The TRAPP complexes are nucleotide exchange factors that play essential roles in membrane traffic and autophagy. TRAPPII activates Rab11, and TRAPPIII activates Rab1, with the two complexes sharing a core of small subunits that affect nucleotide exchange but being distinguished by specific large subunits that are essential for activity in vivo. We report a cryo‐EM structure of the entire Drosophila TRAPPIII complex. The TRAPPIII‐specific subunits TRAPPC8 and TRAPPC11 hold the catalytic core like a pair of tongs, with TRAPPC12 and TRAPPC13 positioned at the joint between them.

The overall shape of the complex is that of two arched arms connected at one vertex with TRAPPC12 and TRAPPC13, and then spreading apart to hold the core between their other ends like a pair of tongs. Overall, we were able to model the core, and the N‐terminal halves of TRAPPC8 and TRAPPC11. The C‐terminal halves of these subunits, along with TRAPPC12 and TRAPPC13, were unmodelled as although helices were recognisable in many regions, the sequences could not be attributed. The primary interactions between the core and the arms are via binding of TRAPPC2 and TRAPPC2L to TRAPPC8 and TRAPPC11, respectively. Two additional points of interaction between the arms and the core are visible in the TRAPPIII map as indicated by continuous densities between the flat surface of the core and the middle regions of both TRAPPC8 and TRAPPC11. TRAPPC8 is linked to density formed by the connection of the first two α‐helices of TRAPPC3b and TRAPPC5. Similarly, density from TRAPPC11 connects to a region formed by the first two α‐helices of TRAPPC3a and TRAPPC6. We detected 146 total cross‐links, and 75 of them mapped to residues present in the structural model—32 cross‐links were inter‐molecular and 43 intra‐molecular. None of these cross‐links exceeded the maximum distance constraint for disuccinimidyl dibutyric urea (DSBU) of ~30 Å, thus providing good validation for the atomic model of the TRAPPIII complex (Appendix Fig S5B and Table EV1). The TRAPPC8 arm is positioned such that it would contact Rab1 that is bound to the core, indicating how the arm could determine the specificity of the complex.

> DNLRHFVQDYAVRALIPYIEHLVAILAEGVTNKKGVSKSLLSATKRWFVTSKPGAGANNQNAVIYTNESAELQTRKLGDLYFMFGHYNLAFQSYHQAKRDFNADSAWQYYAGALEMAALSAFMLGTAQRKTYDYMEDAIVCYLTVCKLQQFATRATLLSMECLKTARLYSEVAKQLIRMTNEESDLRSALLLEQAAYCFLVTQPPMHRKYAFHIVLAGNRYSRAGQRKHAYRCYRQAYQVFQKREWSLAEDHIQYTVAKQAYMLKQLEEASRSFAHLLRPGSLQSAQQQTSFLKEYIQTQNELVKRS;> MTMDATALPSELLVTPQPLVGFCGLDTARVSVHKAVWEAFSGSLQRKAADRAAVQYKLLPPNYEFPVAKPKRASYEWYHPKGILKRNWMLKHLHVLPSVVVLFQDMEWNDLQWTEKQVQCAAIVQALKNTLQERNTRLCLVLLQRAAPLPPGEDLLAAERAASLTNACGITSKMLFILPHTEHLTGYALRLESAFLDMAQSYYALMSKRIRNHRDQLTAAHTSLKIRHQFKLGFVAEMRQDFSTGQKHYFQAYANLDEIRINDGNCLEIKTLAGFLNYKICRLMFKLKTPRDAINQFIIHVEKHKSRVGFKDLAFEHHAWLSTQHSVFAELFCEAIKNGLPALQTQHPGIYYHKAAEFVMKRRDAAMEAYAAMQASSEATPTPIQNPLSLYTEFFGIRAVKTGDLVAEQQANMQLCDQERSYNHSAAIIALLSQAMAQFKIYKCLRFRKKLAIDMAEEYLKSGDHAKALTLYSLMLPDYRQEKWTTIFTDVLLKTLRCALLSGSVADYIACSVEALSLRHQSDQSERILILENLWQVFQGVPPMPKTQLTPEAQALWTSALANVKSPIQIDLDKVNDVVEMCATFERVQLSNDDLLQLQLIVRVLTDIPLRIRSFHVILADAGNPQNSYKLEALKYFCFPTLTQLRGQKQPDDEQLENPSQEPKNFEKNMRLEPGSYYQLFCSTEAQQFHENTQLRIVRLEAHMGTDQVAALLTCSSN;>[2x]MSRQASRLDAKKVNSEFLTLTYGALVTQMLRDFENAEDVNKQLERIGYNMGMRLIEDFLARTSAPRCLEMRETADRIQQAFRIYLNIQPTISNWSPASDEFSLVFDSNPLTEFVELPPDLTNLRYSAILSGCIRGALEMVQLEVQCWFVQDQLKGDNVTELRVKFVRRLEEVIPAGED;> MSEEILFDCLHAEIVNYCLDSNKEHDLATLEYIGFTTGYRLIERLTREVSRFKDELETMKFICTDFWMLIYKKQVDNLRTNNHGMYVVQDKAFRFLTRISPGTKQLEHAPKFVAFTCGLVRGALSNLGINSTVTAEVQSIPACKFHIEVNRN;> MTIFNLYIFDKFGTLLHYAEWNRTKKSGITREEEAKLTYGMLFSIKSFVSKISPHDPKEGFLYYKTNRYALHYLETPSGLKFVLNTDTTAINVKELLQQLYAKVWVEFVVRDPLWTPGTVVTSELFQSKLDEFVRQSPIFGIRNI;> MIIYGVYIVSKSGGLIFNLDNNVPRIEHEKTFTYPLDLVLDYDSKKVSVSFNRKDGINVGHVLVAVNGMPVNGVTLDDGRDVRTTLDAPENYPINLKFSRPKMTTNEKIFLASMFYPLFAIASQLSPEPKSSGIEILEADTFTLHCFQTLTGIKFIIISETGLNGIDLLLRKVYELYSDYVLKNPFYSLEMPIRCELFDNKLQELLAQVEKTGISNIDK;> MSTYYFVIVGQNDNPIYEKEFSTVNKELRKEDHRHLTQFIAHAALDLVDEHKWKTANMQLKSIDRFNQWFVSAFITASQIRFIIVHDNKNDEGIKNFFNEMYDTYIKNSMNAFYRINTPIKSPMFEKKSEIFGRKYLLS;> MEKLEALKISSMRPRSNILDRPLSKGKTEVSQSIVALLFSEIVQYSQSRVFTVPELQTRLHDLGQDVGTRIIDLYFVRERSSKRETKLTQMLLFVKTTVWKNLFGKEAEKLEHANDDERTYYIIEKEPLVNTFISVPKDKGSLNCANFTAGIVEAVLTNCGFPCKVTAHWHKGTTYMVKFEDFVIARDKQMEEK;> MAFCIAVIGKDNAPLYLTTSDMEQELELQYHVNAALDVVEEKCLIGKGAPESKELYLGLLYSTENHKIYGFVTNTRVKFIVVIDSSNVALRENEVRAIFRNLHLLYTDAICNPFYIPGESLTSKKFDRAVQKLMSGTA>[8x]SAAATQAVPAPNQQPEVFCNQIFINNEWHDAVSRKTFPTVNPSTGEVICQVAEGDKEDVDKAVKAARAAFQLGSPWRRMDASHRGRLLNRLADLIERDRTYLAALETLDNGKPYVISYLVDLDMVLKCLRYYAGWADKYHGKTIPIDGDFFSYTRHEPVGVCGQIIPWNFPLLMQAWKLGPALATGNVVVMKVAEQTPLTALYVANLIK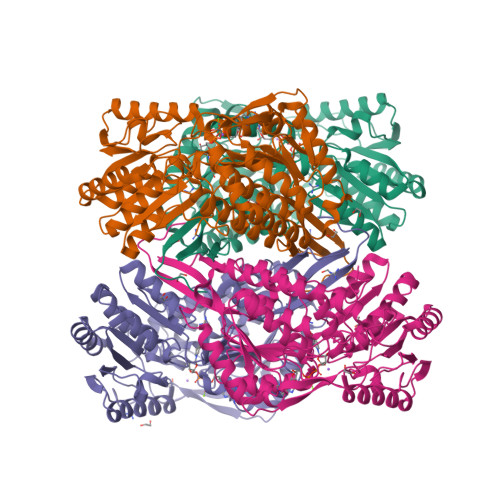EAGFPPGVVNIVPGFGPTAGAAIASHEDVDKVAFTGSTEIGRVIQVAAGSSNLKRVTLELGGKSPNIIMSDADMDWAVEQAHFALFFNQGQCSCAGSRTFVQEDIYDEFVERSVARAKSRVVGNPFDSKTEQGPQVDETQFKKILGYINTGKQEGAKLLCGGGIAADRGYFIQPTVFGDVQDGMTIAKEEIFGPVMQILKFKTIEEVVGRANNSTYGLAAAVFTKDLDKANYLSQALQAGTVWVNCYDVFGAQSPFGGYKMSGSGRELGEYGLQAYTEVKTVTVKVPQKNS D-ERITADENINE | C9 H11 N5 O4 | 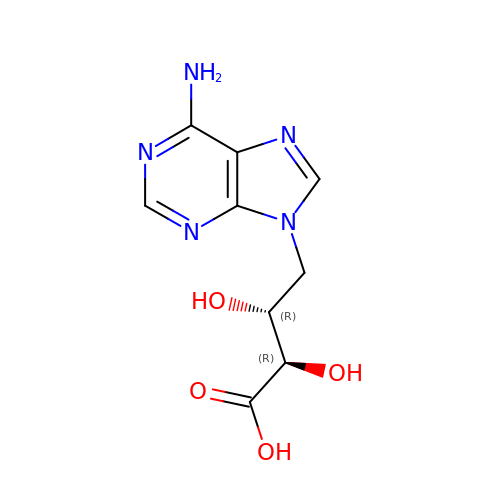LIEMBEWXEZJEEZ-INEUFUBQSA-N> HHMLHLLEQIRAYCE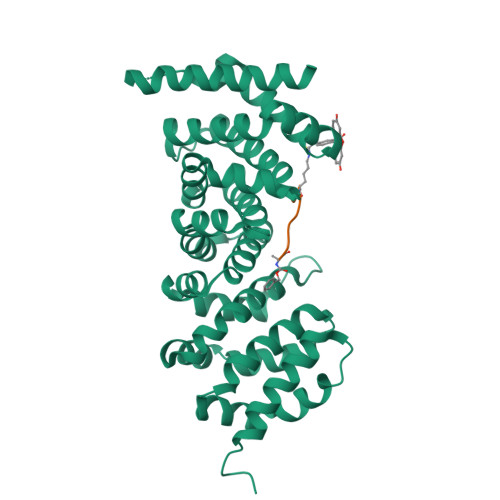TCWEWQEAHEPGMDQDKNPMPAPVEHQICPAVCVLMKLSFDEEHRHAMNELGGLQAIAELLQVDCEMYGLTNDHYSITLRRYAGMALTNLTFGDVANKATLCSMKGCMRALVAQLKSESEDLQQVIASVLRNLSWRADVNSKKTLREVGSVKALMECALEVKKESTLKSVLSALWNLSAHCTENKADICAVDGALAFLVGTLTYRSQTNTLAIIESGGGILRNVSSLIATNEDHRQILRENNCLQTLLQHLKSHSLTIVSNACGTLWNLSARNPKDQEALWDMGAVSMLKNLIHSKHKMIAMGSAAALRNLMANRPAKYK;> XAGESLYEKX> DWVVAPISVPENGKGPFPQRLNQLKSNKDRDTKIFYSITGPGADSPPEGVFAVEKETGWLLLNKPLDREEIAKYELFGHAVSENGASVEDPMNISIIVTDQNDHKPKFTQDTFRGSVLEGVLPGTSVMQVTATDEDDAIYTYNGVVAYSIHSQEPKDPHDLMFTIHRSTGTISVISSGLDREKVPEYTL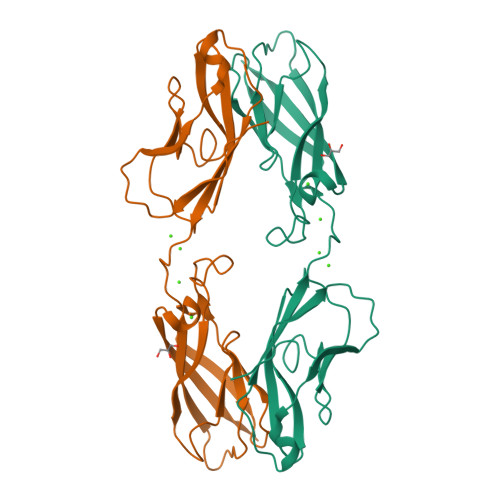TIQATDMDGDGSTTTAVAVVEILDANDNAPMFDPQKYEAHVP>[2x]NPCCSHPCQNRGVCMSVGFDQYKCDCTRTGFYGENCSTPEFLTRIKLFLKPTPNTVHYILTHFKGFWNVVNNIPFLRNAIMSYVLTSRSHLIDSPPTYNADYGYKSWEAFSNLSYYTRALPPVPDDCPTPLGVKGKKQLPDSNEIVEKLLLRRKFIPDPQGSNMMFAFFAQHFTHQFFKTDHKRGPAFTNGLGHGVDLNHIYGETLARQRKLRLFKDGKMKYQIIDGEMYPPTVKDTQAEMIYPPQVPEHLRFAVGQEVFGLVPGLMMYATIWLREHNRVCDVL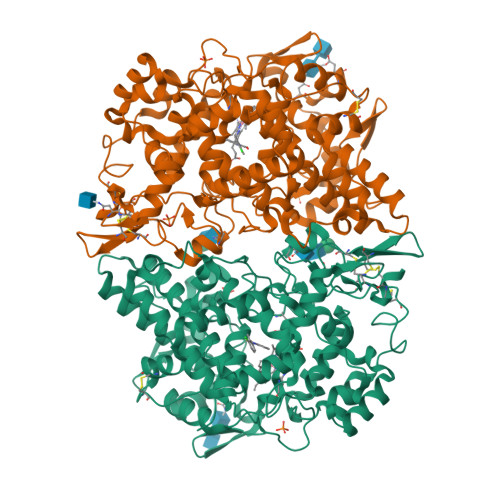KQEHPEWGDEQLFQTSRLILIGETIKIVIEDYVQHLSGYHFKLKFDPELLFNKQFQYQNRIAAEFNTLYHWHPLLPDTFQIHDQKYNYQQFIYNNSILLEHGITQFVESFTRQIAGRVAGGRNVPPAVQKVSQASIDQSRQMKYQSFNEYRKRFMLKPYESFEELTGEKEMSAELEALYGDIDAVELYPALLVEKPRPDAIFGETMVEVGAPFSLKGLMGNVICSPAYWKPSTFGGEVGFQIINTASIQSLICNNVKGCPFTSFSVP The mycobacterial repressor, DarR, a TetR family regulator (TFR), was the first transcription regulator shown to bind c-di-AMP. Recently, DarR, a 201 residue, TFR regulator of a putative MDR transporter, Ms5347, in Mycobacteria was discovered and represents the focus of this work. Structures of TFR proteins reveal that they share a two-domain architecture with an N-terminal DNA-binding domain and a C-terminal inducer binding/dimerization domain. The DarR N-terminal domain consists of helices 1-3 and the dimer domain is comprised of helices α4-α9. In DarR, dimerization is mediated by helices α8 and α9, which interact with α8´ and α9´ (where the prime indicates the other subunit in the dimer) to form a four-helix bundle dimerization module.

We next obtained the structure of the Rhodococcus sp. USK13 DarR-cAMP complex to 1.44 Å resolution. The structure revealed clear density for cAMP molecules bound at each dimer interface, in the same location bound by c-di-AMP. Unlike c-di-AMP, the cAMP appears to be tightly bound to DarR; the B-factors (ave) for the cAMP is 33.5 Å2 compared to 22.6 Å2 for the protein and 36.0 Å2 for water molecules. Interestingly, in this structure the cAMP is rotated ~90 relative to the nucleotides in the c-di-AMP bound structure. Nonetheless, the contacts to the cAMP are provided by the same sets of residues that bind c-di-AMP. The Arg165 side chain contacts both the cAMP ribose and phosphate groups in the DarR-cAMP complex. The cAMP adenine N1 and N6 atoms are read by hydrogen bonds from Gln184 while the adenine N6 and N7 atoms are specified by the backbone carbonyl and amide nitrogen atoms of Arg179. Finally, the side chains of DarR residues Trp177, Tyr178, Ile181 and Leu192 make hydrophobic interactions with the cAMP adenine moiety. The distance between recognition helices in the DarR-c-di-AMP and DarR-cAMP structures is ~43 Å indicating that they also adopt structures more similar to the DNA-bound state. Because cAMP interact with residues from both subunits of the DarR dimer, it would be predicted to function as a stabilizer of dimerization.

> GSHMSASAEPESDVKGRILDAAADAFMLRGFANTTIDDIADDVGATAGLIYYHFRSKFDIFLAVYEDGMRRVRERVEPYVGAPGTGRQRLVAMSVAHVENLMIDLGYHHVVHQGVRDQASTALKVRQRDALAALNELRRDYERMFHHVITEGIADGSLRNVDDALATRTLLSNLNAVDVWYRKIEGQTEKEVHDLASQVVDLLIGGIGATAD> DISTVPDETYDALKLDRGKATPKETYEALVKRYKDPAHGAGKGTMGDYWEPIAISIYMDPNTFYKPPVSPKEVAERKDCVECHSDETPVWVRAWKRSTHANLDKIRNLKSDDPLYYKKGKLEEVENNLRSMGKLGEKETLKEVGCIDCHVDVNKKDKADHTKDIRMPTADTCGTCHLREFAERESERDTMVWPNGQWPAGRPSHALDYTANIETTVWAAMPQREVAEGCTMCHTNQNKCDNCHTRHEFSAAESRKPEACATCHSGVDHNNWEAYTMSKHGKLAEMNRDKWNWEVRLKDAFSKGGQNAPTCAACHMEYEGEYTHNITRKTRWANYPFVPGIAENITSDWSEARLDSWVLTCTQCHSERFARSYLDLMDKGTLEGLAKYQEANAIVHKMYEDGTLTGQKTNRPNPPEPEKPGFGIFTQLFWSKGNNPASLELKVLEMAENNLAKMHVGLAHVNPGGWTYTEGWGPMNRAYVEIQDEYTKMQELSALQARVNKLEGKQTSLLDLKGTGEKISLGGLGGGMLLAGALALIGWRKRKQTR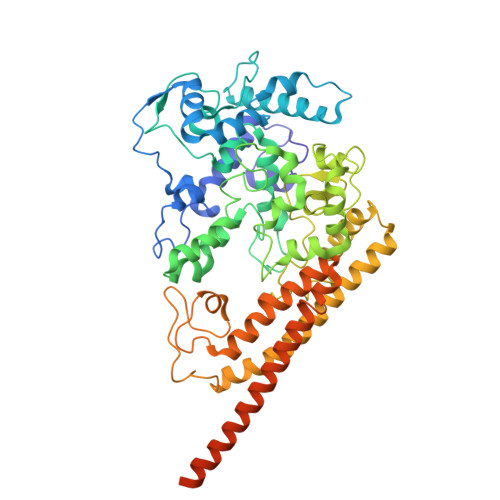A> GAMDGTAAEPRPGAGSLQHAQPPPQPRKKRPEDFKFGKILGEGSFSTVVLARELATSREYAIKILEKRHIIKENKVP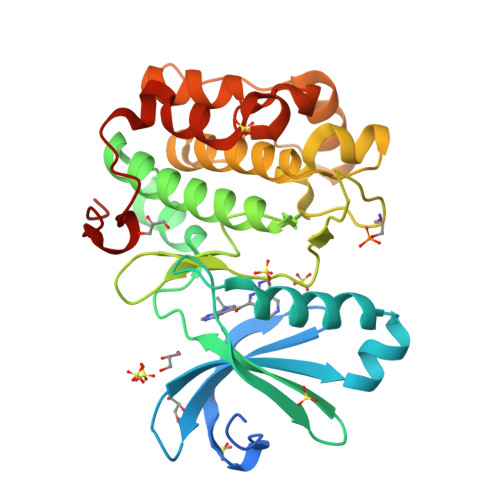YVTRERDVMSRLDHPFFVKLYFTFQDDEKLYFGLSYAKNGELLKYIRKIGSFDETCTRFYTAEIVSALEYLHGKGIIHRDLKPENILLNEDMHIQITDFGTAKVLSPESKQARANSFVGTAQYVSPELLTEKSACKSSDLWALGCIIYQLVAGLPPFRAGNEYLIFQKIIKLEYDFPEKFFPKARDLVEKLLVLDATKRLGCEEMEGYGPLKAHPFFESVTWENLHQQTPPKLT> MMNNKTPLSTQSLIEVKNLSFNRGERVIYDNISLNIRRGQITAIMGPSGTGKTTLLRLIGGQLVPDQGEVLLDGKDIAQMSRQELFAARARMGMLFQSGALFTDMSVYENVAFPIRAHTKLSENLIAE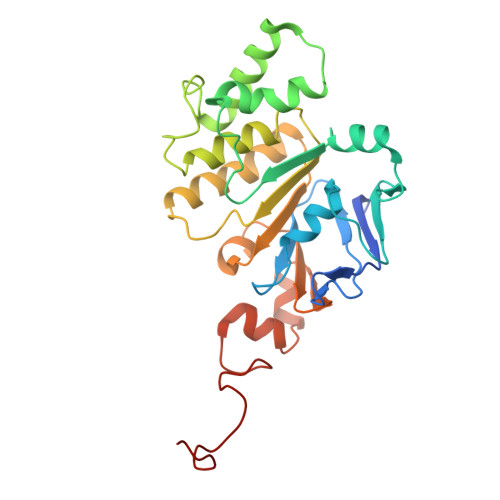LVALKLESVGLRGTEQLMPTELSGGMNRRVALARAIALDPDLIMYDEPFAGQDPIVKGVLTRLIRSLREALDLTTIIVSHDVPETLSIADYIYVVAEGKIQGEGTPEELQAYASPFVKQFLTGSAEGPVEYQFSHQAYLDNEVRP>[2x]MITQEMKDLINNQLAMVATVDAKGQPNIGPKRSMRLWDDKTFIYNENTDGQTRINIEDNGKIEIAFVDRERLLGYRFVGTAEIQTEGAYYEAAKKWAQGRMGVPKAVGIIAVERIFNLQSGANAGKEINSESNKGELNSKLEGKPIPNPLLGLDSTRTGHHHHHH

Hence, spy49_0662 was expressed with a 1.4 kDa C-terminal V5 epitope tag used for Western blotting followed by a His6-tag for immobilized metal ion affinity purification, and the resulting protein was coined as HupZ (heme utilization protein Z). The tagged HupZ is a small-sized protein previously shown to bind heme, and it exhibits a trace heme degrading activity in the presence of NADPH and cytochrome P450 reductase (CPR). This protein shares some protein sequence similarity to the members of the IsdG family. In summary, a comprehensive biochemical, spectroscopic, and structural characterization led us to propose that the observed heme binding in HupZ is through its His6-tag in a sandwiched di-heme complex from two subunits with an oxygen-derived bridging ligand.

Because our UV–vis and rR data suggested a histidine as an axial ligand, we turned our attention to His111 in HupZ, which is the only histidine residue aside from the C-terminal tag. We mutated His111 to probe its potential role in heme binding. The H111A variant was crystallized in the P6522 hexagonal trapezohedral space group, and its structure was solved and refined to 1.98-Å resolution. Comparing the structure of H111A to the wild-type structure, the two superimpose well with an r.m.s.d value of 0.99 Å over 237 Cα carbons, indicating site-directed mutagenesis did not induce an undesired global structural perturbation. The UV–vis spectrum of the heme-bound H111A variant is nearly identical to wild-type HupZ. H111A in complex with heme was EPR silent, as observed in the binary complex of wild-type HupZ, indicating mutation of His111 did not lead to an observable change of the heme-center electronic structure. Since H111A and wild-type HupZ show nearly identical UV–vis, EPR, and rR spectra, His111 is not a heme ligand for HupZ. The difference in SEC between the heme complex of wild-type HupZ and the H111A variant suggests that His111 is exposed to surface or involved in subunit-subunit interactions; and thus, mutating such a polar residue facilitated the formation of high-order oligomer structures. We noted that the H111A variant had similar activity comparable to that of wild-type HupZ, suggesting that His111 does not contribute to the observed activity. The only remaining histidine residues are present in the C-terminal tag; therefore, we conclude that the heme binding to HupZ occurs at His6-tag.> MEHDERTHVPVELRAAGVVLLNERGDILLVQEKGIPGHPEKAGLWHIPSGAVEDGENPQDAAVREACEETGLRVRPVKFLGAYLGRFPDGVLILRHVWLAEPEPGQTLAPAFTDEIAEASFVS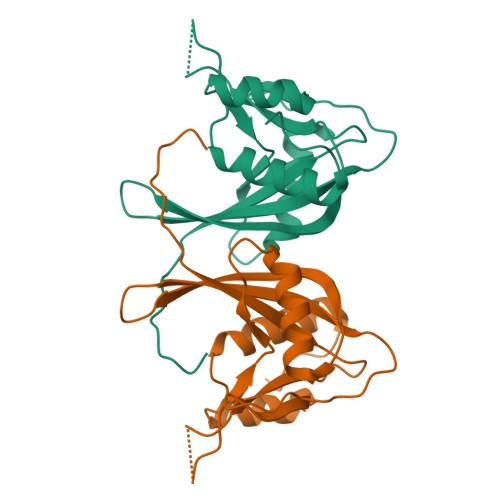REDFAQLYAAGQIRMYQTKLFYADALREKGFPALPV> SHRNEAGHGDLHEILHEAVPLDANEREILELKEDAFAQRRREIETRLRAANGKLADAIAKNPAWSPEVEAATQEVERAAGDLQRATLV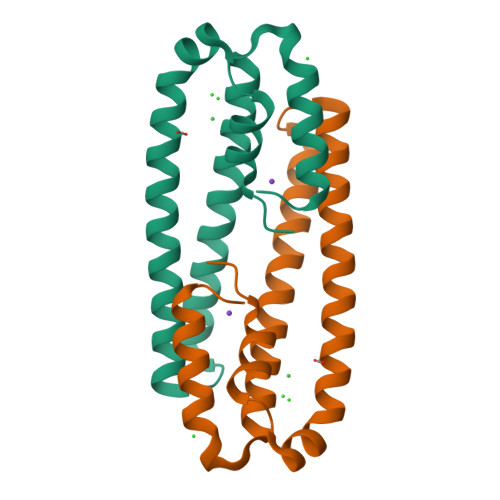HVFEMRAGLKPEHRPAFDRVLIDALRRGSQ>[4x]SHMKYSLSADHHIFAFSKENKPAISVKSGDELEVETMDCFSNQIQSNEDKLDEMDWNRVNPATGPIFVEGAKEGDVLKVKIKKIEVAEKGVLATGKGLGVLGNLMEGLYSKVVDIKDGKVIFNEKLALPVKPMIGVIGVAPKEGSINCGTPGSHGGNMDTTLIAEGAEVYFPVFVEGALLALGDLHALMGDGEVGVSGVEVAGKVLLEVEVIKGLNLKNPVVKTAEVTATIASAESLDKAVEIAVH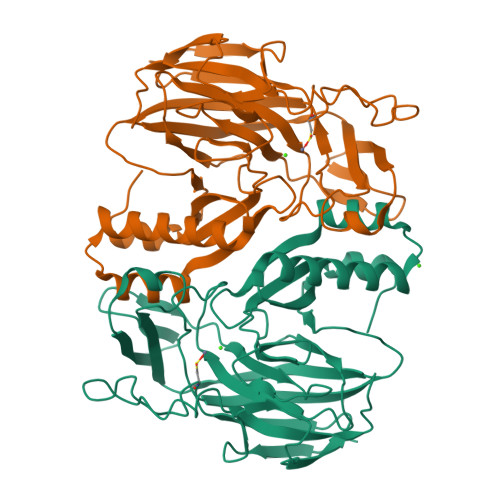DMAELFKKHTDLSTEGIATLFSITGNAQISQVVDPLKTARFSLPNWILESYGIRF> VA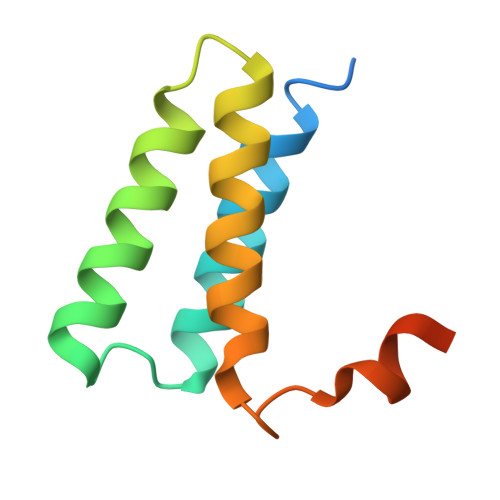CTKEVHMSKMSDVKCTSVVLLSVLQQLRVESSSKLWAQCVQLHNDILLAKDTTEAFEKMVSLLSVLLSMQGAVDINKLCEEMLDNRATLQ> MQKQILTSQKRNMYILSRCKVLVKNGQVCHLHEDGNVYTVPYANTVFIGLAEGTSITNEA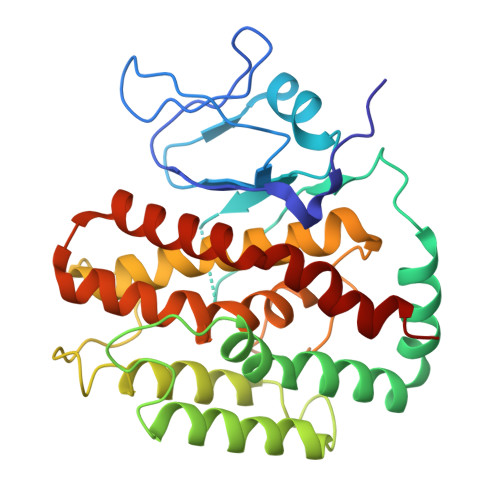MSMLAANGVIVFWTKGGGYDMFAADIICHLPQADYRPTKYMQNWVRLWLDEEKKLSAAKEILKMRVDSLSTHVHDFGVDVENKRVSSIVNKFDKGVTQATSFESLLGHEGTFVKSLYKEYALEYEIEFKRDHKSADNYNKFLTLGNYYAYGIARSSLWALGIDNSFPLLHGSTRRGGLVFDVADIIKTSIILPLAFHAADQGMSNTEFKRSCVAYFDKNDILAYLINNIKRLCMEN>MFESMKPHLAELRQRLAISVLAVFVGFIIAFTFHNAILGWITKPLNNALIQVGKIVEKREMGTWKISGNEHNATLAPSKSPALLSDHAQSAEKLHRTLAEASQATQNPKLQKLLSQAASAAEELARNSRILRKALVKEENLTRQAVNQNLREKSFNGMITTHQVGGAFFVALKVSFFAGILMAMPVILWQLWLFIAPGLYDNEKKMVLPFVVGGSVMFLIGVLFAYYVVTPFGFQFLITFGSFLYTPLINIEDYVGFFTKILIGFGIAFELPVVAYFLALLGLITDKTLKDYFKYAIVIIFLLAAFLTPPDVLTQLLMAAPLILLYGLSILIVHYVNPYKPEEKEDDEEEEEDEFEKAEREFEALEKGSESHESGSENLYFQ[3x];>[3x]MFGMGFSEILVIALVAILFLGPDKLPEAMVQIAKFFNSVRKTINEAKSTFEEELHLKELKEEALSYRQSLSEVGSDISGFKNAISNHTDELQEAIEIARSGMPTDRLNESVDDLLEEDEPTGETSQRPGVTEYKEMARKA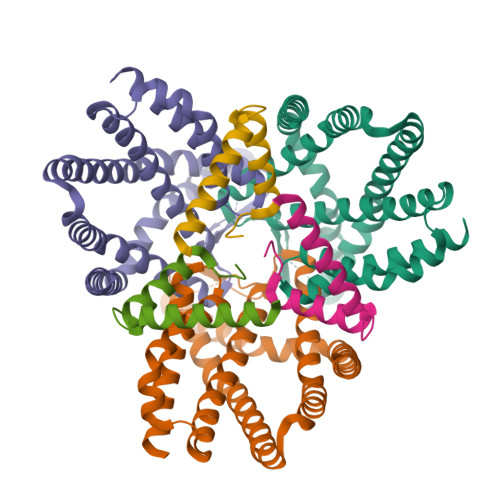LEEAENSAEAQTAETPSVEDKGPESSPKESSRPAGFKHLDNEANAWSHPQFEK>[4x]ATAAQAERTLPKKYGGRFTVTLIPGDGVGKEITDSVRTIFEAENIPIDWETINIKQTDHKEGVYEAVESLKRNKIGLKGLWHTPADQTGHGSLNVALRKQLDIYANVALFKSLKGVKTRIPDIDLIVIRENTEGEFSGLEHESVPGVVESLKVMTRPKTERIARFAFDFAKKYNRKSVTAVHKANIMKLGDGLFRNIITEIGQKEYPDIDVSSIIVDNASMQAVAKPHQFDVLVTPSMYGTILGNIGAALIGGPGLVAGANFGRDYAVFEPGSRHVGLDIKGQNVANPTAMILSSTLMLNHLGLNEYATRISKAVHETIAEGKHTTRDIGGSSSTTDFTNEIINKLSTMHHHHH;>ATVKQPSIGRYTGKPNPSTGKYTVSFIEGDGIGPEISKSVKKIFSAANVPIEWESCDVSPIFVNGLTTIPDPAVQSITKNLVALKGPLATPIGKGHRSLNLTLRKTFGLFANVRPAKSIEGFKTTYENVDLVLIRENTEGE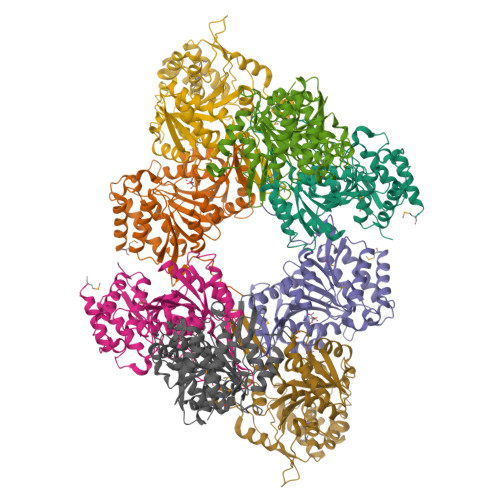YSGIEHIVCPGVVQSIKLITRDASERVIRYAFEYARAIGRPRVIVVHKSTIQRLADGLFVNVAKELSKEYPDLTLETELIDNSVLKVVTNPSAYTDAVSVCPNLYGDILSDLNSGLSAGSLGLTPSANIGHKISIFEAVHGSAPDIAGQDKANPTALLLSSVMMLNHMGLTNHADQIQNAVLSTIASGPENRTGDLAGTATTSSFTEAVIKRL[4x]>[2x]SERFPNDVDPIETRDWLQAIESVIREEGVERAQYLIDQLLAEARKGGVNVAAGTGISNYINTIPVEEQPEYPGNLELERRIRSAIRWNAIMTVLRASKKDLELGGHMASFQSSATIYDVCFNHFFRARNEQDGGDLVYFQGHISPGVYARAFLEGRLTQEQLDNFRQEVHGNGLSSYPHPKLMPEFWQFPTVSMGLGPIGAIYQAKFLKYLEHRGLKDTSKQTVYAFLGDGEMDAPESKGAITIATREKLDNLVF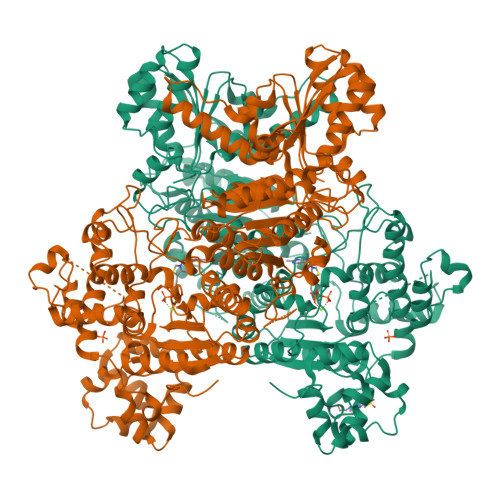VINCNLQRLDGPVTGNGKIINELEGIFEGAGWNVIKVMWGSRWDELLRKDTSGKLIQLMNETVDGDYQTFKSKDGAYVREHFFGKYPETAALVADWTDEQIWALNRGGHDPKKIYAAFKKAQETKGKATVILAHTIKGYGMGDAAEGKNIAHQVKKMNMDGVRHIRDRFNVPVSDADIEKLPYITFPEGSEEHTYLHAQRQKLHGYLPSRQPNFTEKLELPSLQDFGALLEEQSKEISTTIAFVRALNVMLKNKSIKDRLVPIIADEARTFGMEGLFRQIGIYSPNGQQYTPQDREQVAYYKEDEKGQILQEGINELGAGCSWLAAATSYSTNNLPMIPFYIYYSMFGFQRIGDLCWAAGDQQARGFLIGGTSGRTTLNGEGLQHEDGHSHIQSLTIPNCISYDPAYAYEVAVIMHDGLERMYGEKQENVYYYITTLNENYHMPAMPEGAEEGIRKGIYKLETIEGSKGKVQLLGSGSILRHVREAAEILAKDYGVGSDVYSVTSFTELARDGQDCERWNMLHPLETPRVPYIAQVMNDAPAVASTDYMKLFAEQVRTYVPADDYRVLGTDGFGRSDSRENLRHHFEVDASYVVVAALGELAKRGEIDKKVVADAIAKFNIDADKVNPRLA> TMRITKVEVDRKKVLISRDKNGGKLVYENEMQDNTEQIMHHKKSSFYKSVVNKTICRPEQKQMKKLVHGLLQENSQEKIKVSDVTKLNISNFLNHRFKKSLYYFPENSPDKSEEYRIEINLSQLLEDSLKKQQGTFICWESFSKDMELYINWAENYISSKTKLIKKSIRNNRIQSTESRSGQLMDRYMKDILNKNKPFDIQSVSEKYQLEKLTSALKATFKEAKKNDKEINYKLKSTLQNHERQIIEELKENSELNQFNIEIRKHLETYFPIKKTNRKVGDIRNLEIGEIQKIVNHRLKNKIVQRILQEGKLASYEIESTVNSNSLQKIKIEEAFALKFINACLFASNNLRNMVYPVCKKDILMIGEFKNSFKEIKHKKFIRQWSQFFSQEITVDDIELASWGLRGAIAPIRNEIIHLKKHSWKKFFNNPTFKVKKSKIINGKTKDVTSEFLYKETLFKDYFYSELDSVPELIINKMESSKILDYYSSDQLNQVFTIPNFELSLLTSAVPFAPSFKRVYLKGFDYQNQDEAQPDYNLKLNIYNEKAFNSEAFQAQYSLFKMVYYQVFLPQFTTNNDLFKSSVDFILTLNKERKGYAKAFQDIRKMNKDEKPSEYMSYIQSQLMLYQKKQEEKEKINHFEKFINQVFIKGFNSFIEKNRLTYICHPTKNTVPENDNIEIPFHTDMDDSNIAFWLMCKLLDAKQLSELRNEMIKFSCSLQSTEEISTFTKAREVIGLALLNGEKGCNDWKELFDDKEAWKKNMSLYVSEELLQSLPYTQEDGQTPVINRSIDLVKKY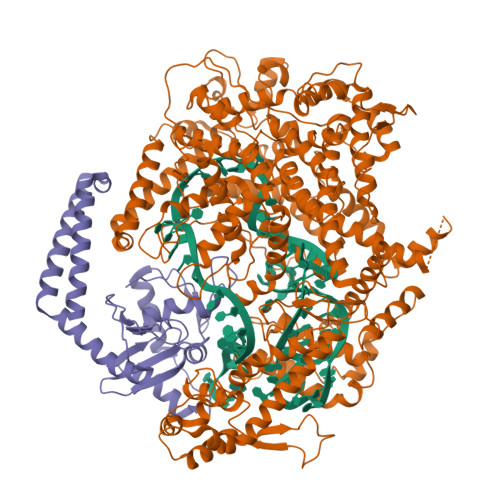GTETILEKLFSSSDDYKVSAKDIAKLHEYDVTEKIAQQESLHKQWIEKPGLARDSAWTKKYQNVINDISNYQWAKTKVELTQVRHLHQLTIDLLSRLAGYMSIADRDFQFSSNYILERENSEYRVTSWILLSENKNKNKYNDYELYNLKNASIKVSSKNDPQLKVDLKQLRLTLEYLELFDNRLKEKRNNISHFNYLNGQLGNSILELFDDARDVLSYDRKLKNAVSKSLKEILSSHGMEVTFKPLYQTNHHLKIDKLQPKKIHHLGEKSTVSSNQVSNEYCQLVRTLLTMK;> MIYYIKDLKVKGKIFENLMNKEAVEGLITFLKKAEFEIYSRENYSKYNKWFEMWKSPTSSLVFWKNYSFRCHLLFVIEKDGECLGIPASVFESVLQIYLADPFAPDTKELFVEVCNLYECLADVTVVEHFEAEESAWHKLTHNETEVSKRVYSKDDDELLKYIPEFLDTIATNKKSQKYNQIQGKIQEINKEIATLYESSEDYIFTEYVSNLYRESAKLEQHSKQILKE> MQILFND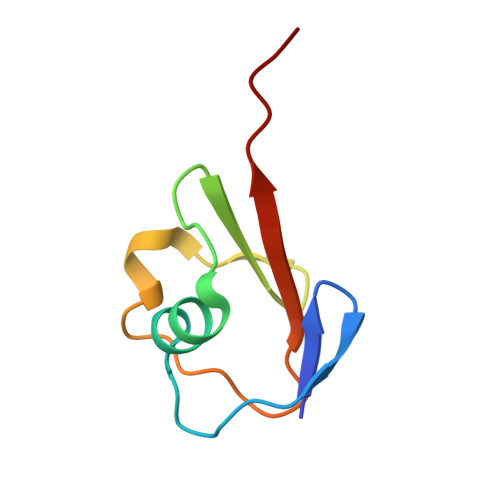QAMQCAAGQTVHELLEQLDQRQAGAALAINQQIVPREQWAQHIVQDGDQILLFQVIAGG>[2x]MGDQRFGDLVFRQLAPNVWQHTSYLDMPGFGAVASNGLIVRDGGR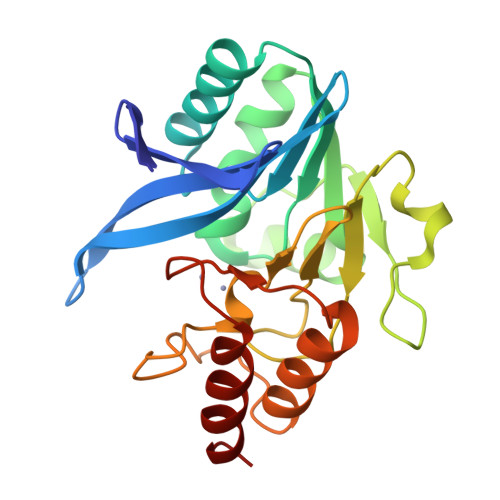VLVVDTAWTDDQTAQILNWIKQEINLPVALAVVTHAHQDKMGGMDALHAAGIATYANALSNQLAPQEGLVAAQHSLTFAANGWVEPATAPNFGPLKVFYPGPGHTSDNITVGIDGTDIAFGGCLIKDSKAKSLGNLGDADTEHYAASARAFGAAFPKASMIVMSHSAPDSRAAITHTARMADKLR2-[(~{E},6~{S},10~{S})-6,10-bis(oxidanyl)undec-1-enyl]-4,6-bis(oxidanyl)benzoic 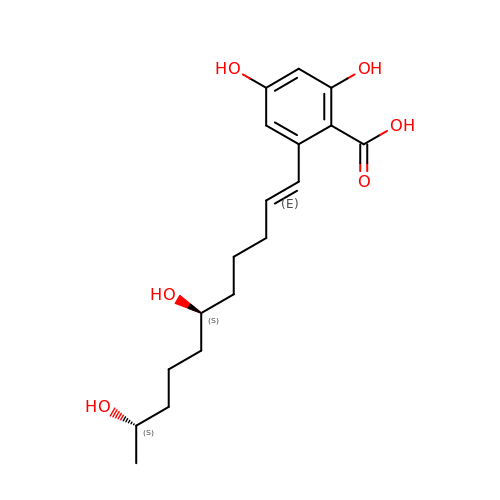acid | C18 H26 O6 | RSYOKTAWJDYBRR-PMRAARRBSA-N>MGKPFTLSLSSLCLLLLSSACFAISSSKLNECQLNNLNALEPDHRVESEGGLIQTWNSQHPELKCAGVTVSKLTLNRNGLHLPSYSPYPRMIIIAQGKGALGVAIPGCPETFEEPQEQSNRRGSRSQKQQLQDSHQKIRHFNEGDVLVIPPGVPYWTYNTGDEPVVAISLLDTSNFNNQLDQTPRVFYLAGNPDIEYPETMQQQQQQKSHGGRKQGQHQQEEEEEGGSVLSGFSKHFLAQSFNTNEDIAEKLQSPDDERKQIVTVEGGLSVISPKWQEQQDEDEDEDEDDEDEQIPSHPPRRPSHGKREQDEDEDEDEDKPRPSRPSQGKREQDQDQDEDEDEDE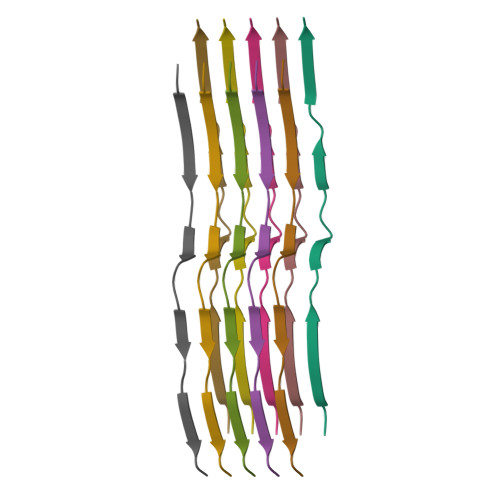DQPRKSREWRSKKTQPRRPRQEEPRERGCETRNGVEENICTLKLHENIARPSRADFYNPKAGRISTLNSLTLPALRQFQLSAQYVVLYKNGIYSPHWNLNANSVIYVTRGQGKVRVVNCQGNAVFDGELRRGQLLVVPQNFVVAEQAGEQGFEYIVFKTHHNAVTSYLKDVFRAIPSEVLAHSYNLRQSQVSELKYEGNWGPLVNPESQQGSPRVKVA[10x]> YKVERNPPAFTELQLPRYIMAGFPVCPKLSLEFGDPASSLFRWYKEAKPGAAGSSWTETDVEERVYTPSNADIGLRLKLHCTPGDGQRFGHSRELESVCVVEAGPGTCTFDHRHLYTKKVTEDALIRTVSYNILADTYAQTEFSRTVLYPYCAPYALELDYRQNLIQKELTGYNADVICLQEVDRAVFSDSLVPALEAFGLEGVFRIKQHEGLATFYRKSKFSLLSQHDISFYEALESDPLHKELLEKLVLYPSAQEKVLQRSSVLQVSVLQSTKDSSKRICVANTHLYW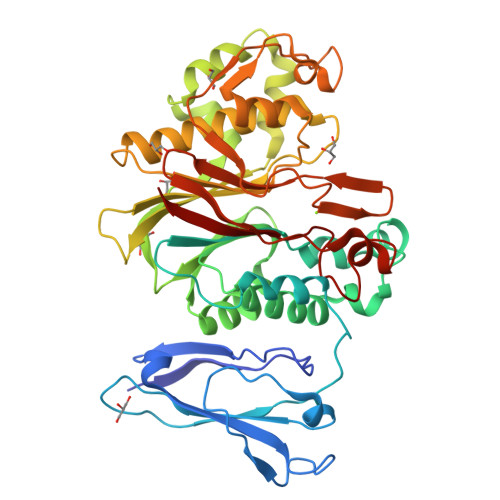HPKGGYIRLIQMAVALAHIRHVSCDLYPGIPVIFCGDFNSTPSTGMYHFVINGSIPEDHEDWASNGEEERCNMSLTHFFKLKSACGEPAYTNYVGGFHGCLDYIFIDLNALEVEQVIPLPSHEEVTTHQALPSVSHPSDHIALVCDLKWK> GSGASKLRAVLEKLKLSRDDISTAAGMVKGVVDHLLLRLKCDSAFRGVGLLNTGSYYEHVKISAPNEFDVMFKLEVPRIQLEEYSNTRAYYFVKFKRNPKENPLSQFLEGEILSASKMLSKFRKIIKEEINDIKDTDVIMKRKRGGSPAVTLLISEKISVDITLALESKSSWPASTQEGLRIQNWLSAKVRKQLRLKPFYLVPKHAKEGNGFQEETWRLSFSHIEKEILNNHGKSKTCCENKEEKCCRKDCLKLMKYLLEQLKERFKDKKHLDKFSSYHVKTAFFHVCTQNPQDSQWDRKDLGLCFDNCVTYFLQCLRTEKLENYFIPEFNLFSSNLIDKRSKEFLTKQIEYERNNEFPVFDEF

Recent studies identified cyclic GMP-AMP synthase (cGAS) as a cytosolic DNA PRR, and its product, cyclic GMP-AMP (cGAMP), binds to STING as a second messenger, resulting in the activation of the STING-dependent IRF3 pathway. In the presence of dsDNA, cGAS produces cGAMP from GTP and ATP, which activates STING as a second messenger. The structure of cGAS adopts the typical nucleotidyl transferase fold, consisting of the N-terminal α/β core and the C-terminal helix bundle. An HCCC type zinc finger (ZnF) exists between the N-terminal core and the C-terminal bundle.

To address the mechanism of immune activation by cGAS, we expressed, purified, and crystallized human cGAS (residues 161–522), including the active site and the double-stranded DNA (dsDNA) binding region. The crystals diffracted to 1.95 Å resolution and belonged to the orthorhombic space group P2 12 12, with unit-cell dimensions a = 123.5, b = 48.31, and c = 59.57 Å. The catalytic Glu225, Asp227, and Asp319 residues are located on the centrally-twisted β sheets. Despite our high resolution structure, electron densities were not observed for the regions between β1 and β2, and between α2 and β7 near the catalytic pocket, indicating their structural flexibility. A zinc ion is coordinated by the side chains of His390, Cys396, Cys397 and Cys404, and forms a protruding loop structure. In our structure, Leu174 is oriented toward the solvent, as seen in the mouse and porcine apo structures, and the catalytic pocket is partially disordered. These observations suggested that a similar structural change would occur in human cGAS upon DNA binding for catalytic activation. The concave DNA binding cleft of human cGAS is composed of a positively charged cluster of lysine and arginine residues, mainly from α1, α4, and α5. In contrast, the ZnF in the human structure forms a partial helix with Lys400 (equivalent to Ser388 and Asp377 in the mouse and porcine proteins, respectively), which is exposed towards the solvent, suggesting an additional interaction between the ZnF of human cGAS and dsDNA. Our structure of the human cGAS apo form resembles those of the mouse (69% sequence identity, r.m.s. deviation = 1.40 Å for 315 Cα atoms) and porcine (74% sequence identity, r.m.s. deviation = 1.11 Å for 312 Cα atoms) apo proteins.>[4x]MERQVLLSEPEEAAALYRGLSRQPALSAACLGPEVTTQYGGRYRTVHTEWTQRDLERMENIRFCRQYLVFHDGDSVVFAGPAGNSVETRGELLSRESPSGTMKAVLRKAGGTGTAEEKQFLEVWEKNRKLKSFNLSALEKHGPVYEDDCFGCLSWSHSETHLLYVADKKRPKAESFFQTKALDVTGSDDEMARTKKPDQAIKGDQFLFYEDWGENMVSKSTPVLCVLDIESGNISVLEGVPESVSPGQAFWAPGDTGVVFVGWW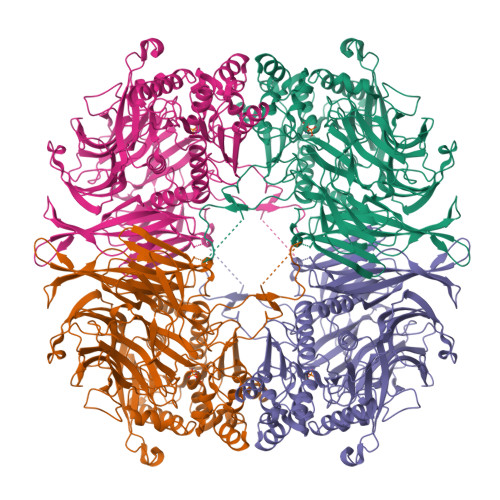HEPFRLGIRFCTNRRSALYYVDLTGGKCELLSDESVAVTSPRLSPDQCRIVYLRFPSLVPHQQCGQLCLYDWYTRVTSVVVDIVPRQLGEDFSGIYCSLLPLGCWSADSQRVVFDSPQRSRQDLFAVDTQMGSVTSLTAGGSGGSWKLLTIDRDLMVVQFSTPSVPPSLKVGFLPPAGKEQAVSWVSLEEAEPFPDISWSIRVLQPPPQQEHVQYAGLDFEAILLQPSNSPEKTQVPMVVMPHGGPHSSFVTAWMLFPAMLCKMGFAVLLVNYRGSTGFGQDSILSLPGNVGHQDVKDVQFAVEQVLQEEHFDAGRVALMGGSHGGFLSCHLIGQYPETYSACVVRNPVINIASMMGSTDIPDWCMVEAGFSYSSDCLPDLSVWAAMLDKSPIKYAPQVKTPLLLMLGQEDRRVPFKQGMEYYRVLKARNVPVRLLLYPKSTHALSEVEVESDSFMNAVLWLCTHLGS6-AMINO-3-METHYLPURINE | C6 H8 N5 | 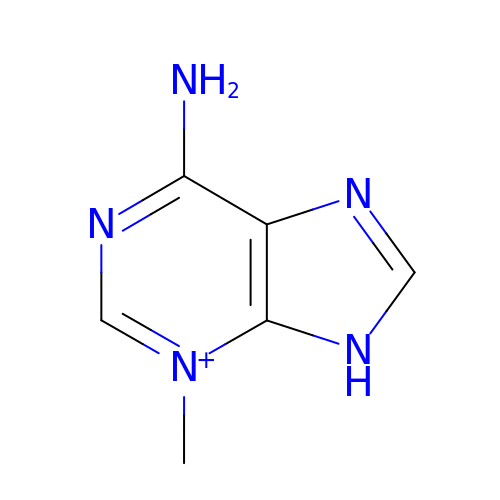YLIQVEPMZVVUEK-UHFFFAOYSA-O3,5-DIMETHYL-1H-PYRAZOLE-4-CARBOXYLIC ACID ETHYL ESTER | C8 H12 N2 O2 | 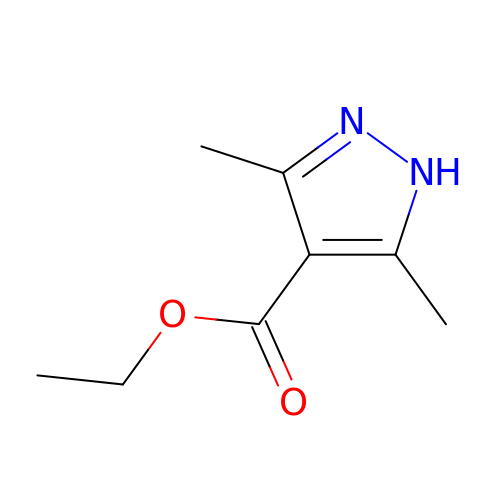BCKARVLFIJPHQU-UHFFFAOYSA-N> X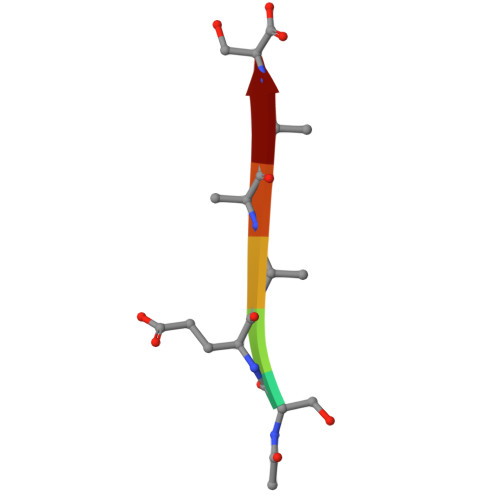SEAAAS>[6x]PLLKFDLFYGRTDAQIKSLLDAAHGAMVDAFGVPANDRYQTVSQHRPGEMVLEDTGLGYGRSSAVVLLTVISRPRSEEQKV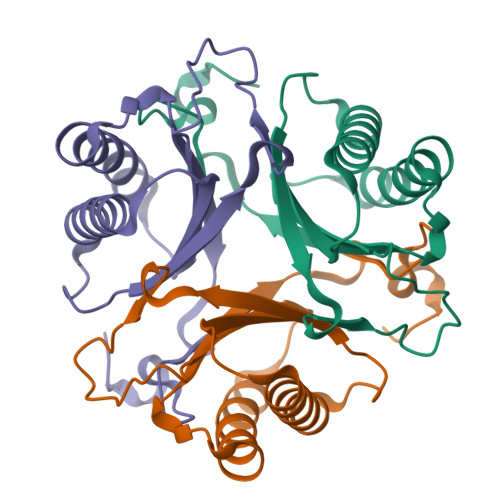CFYKLLTGALERDCGISPDDVIVALVENSDADWSFGRGRAEFLTGDLVG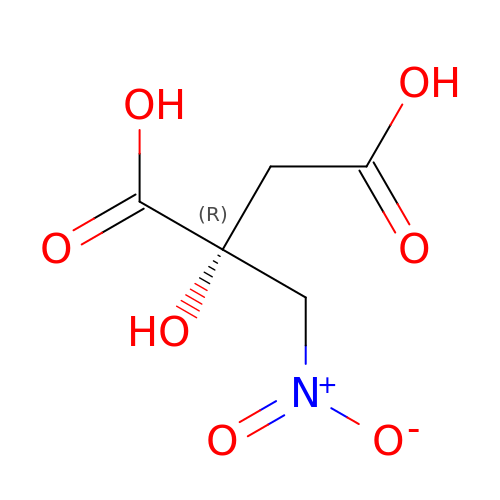2-HYDROXY-2-NITROMETHYL SUCCINIC ACID | C5 H7 N O7 | MTIGFRIXIPBOPZ-RXMQYKEDSA-N> MGSSHHHHHHSQDPQDLNFGQVVADVLCEFLEVAVHLILYVREVYPVGIFQKRKKYNVPVQMSCHPELNQYIQDTLHCVKPLLEKNDVE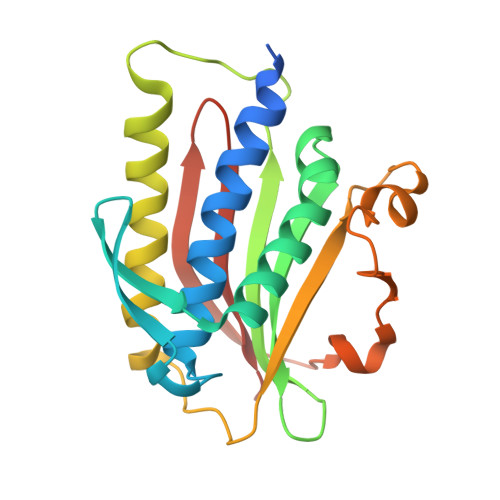KVVVVILDKEHRPVEKFVFEITQPPLLSISSDSLLSHVEQLLAAFILKISVCDDVLDHNPPGCTFTVLVHTREAATRNMEKIQVIKDFPWILADEQDVHMHDPRLIPLKTMTSDILKMQLYVEERAHKGS> PKVSVLITVTGVDQPGVTATLFEVLSRHGVELLNVEQVVIRHRLTLGVLVCCPADVADGPALRHDVEAAIRKVGL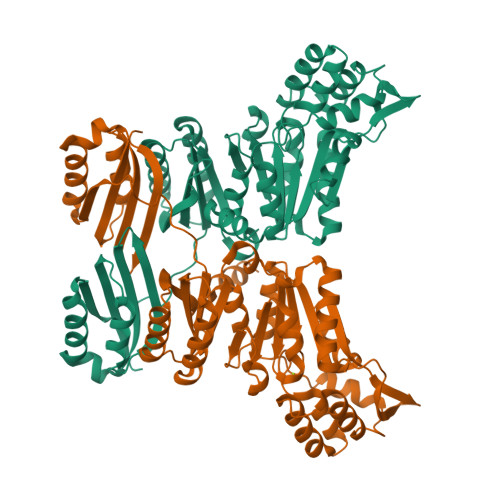DVSIERSDDVPIIREPSTHTIFVLGRPITAAAFGAVAREVAALGVNIDLIRGVSDYPVIGLELRVSVPPGADGALRTALNRVSSEEHVDVAVEDYTLERRAKRLIVFDVDSTLVQGEVIEMLAAKAGAEGQVAAITDAAMRGELDFAQSLQQRVATLAGLPATVIDEVAGQLELMPGARTTLRTLRRLGYACGVVSGGFRRIIEPLAEELMLDYVAANELEIVDGTLTGRVVGPIIDRAGKATALREFAQRAGVPMAQTVAVGNGANNIDMLAAAGLGIAFNAKPALREVADASLSHPYLDTVLFLLGVTRGEIEAADAID>GSHMEVVNMKAKEIIEFIETFAPKDLAIEGD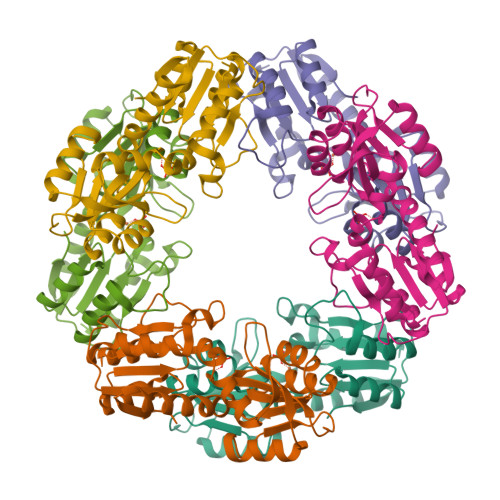NIGLQVGDNLDKEIKKLGIALDPSLSVIKKAEKEGVDFLFTHHPLLKDPIRNFTGVIYKKLKILMENDIILYSAHTNLDICKNGLNDALAELYNLENPKPLYDNGLGRVGIFKGSFEEFLEITKKYIHKNPIVVKSKEVDDNFKLAVLSGYGLSQSSIKYVAEKADVYLSGDLTHHSKILAEELGLVVVDATHYSTEVFGLKKFKEFLSSNLDLEIISLDF[12x]> MVASVSIQNVVKRYDKTTVVHGVSLDIEPGEFVVLVGPSGCGKSTTLRMVAGLEEISGGTIRIDGRVINDLAPKDRDVAMVFQNYALYPHLNVRDNISFGLRLKRTKKSVIDAAVKTAADILG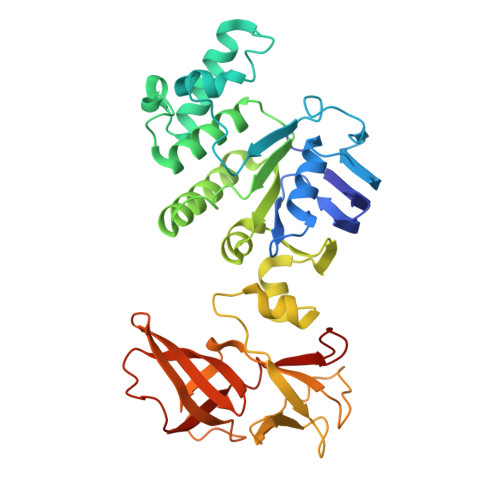LQPLLERKPSDLSGGQRQRVAMGRAIVRDPKVFLFDQPLSNLDAKLRTQMRAEIKRLHQRLGTTVIYVTHDQVEAMTLADRIVVMRDGLIEQIGKPMDLFLHPANTFVASFIGSPPMNLMPARIAVDSTQHVELNGGNRISLLPRAGTHLAPGQEVVFGIRPEDVTLDGVEGSERAQIKATVDIVEPLGSESILHATVGDHSLVVKVGGLNEVHPGDPVTLHVDLTRVHLFDAQSQASIY> MKELNDLEKKYNAHIGVYALDTKSGKEVKFNSDKRFAYASTSKAINSAILLEQVPYNKLNKKVHINKDDIVAYSPILEKYVGKDITLKALIEASMTYSDNTANNKIIKEIGG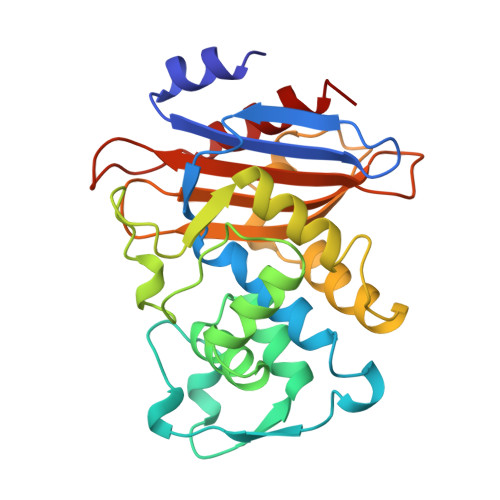IKKVKQRLKELGDKVTNPVRYEIELMYYSPKSKKDTSTPAAFGKTLNKLIANGKLSKENKKFLLDLMLNNKSGDTLIKDGVPKDYKVADKSGQAITYASRNDVAFVYPKGQSEPIVLVIFTNKDNKSDKPNDKLISETAKSVMKEF2-(2-(2-(2-(2-(2-ETHOXYETHOXY)ETHOXY)ETHOXY)ETHOXY)ETHOXY)ETHANOL 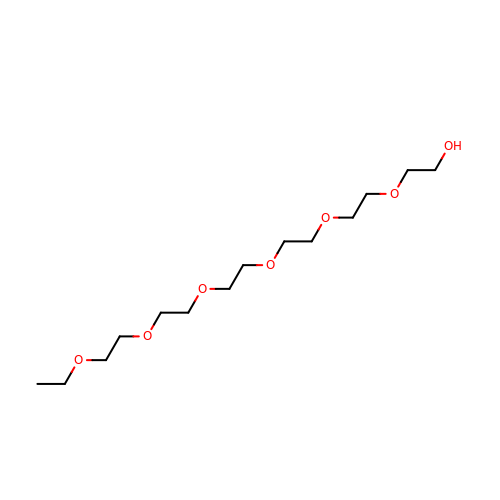| C14 H30 O7 | UKXKPKBTMYNOFS-UHFFFAOYSA-N> GAGCAGACCAG;> ACGCCACTCA;> CTCGT;> TCTGAGTG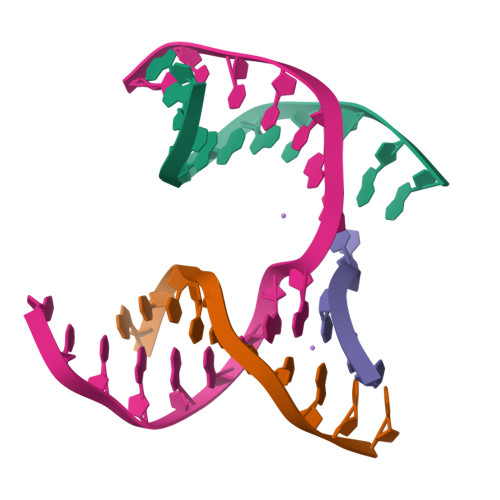GGGTCTGC>MGHHHHHHMKFGPETIIHGDCIEQMNALPEKSVDLIFADPPYNLQLGGDLLRPDNSKVDAVDDHWDQFESFAAYDKFTREWLKAARRVLKDDGAIWVIGSYHNIFRVGVAVQDLGFWILNDIVWRKSNPMPNFKGTRFANAHETLIWASKSQNAKRYTFNYDALKMANDEVQMRSDWTIPLCTGEERIKGADGQKAHPTQKPEALLYRVILSTTKPGDVILDPFFGVGTTGAAAKRLGRKFIGIEREAEYLEHAKARIAKVVPIAPEDLDVMGSK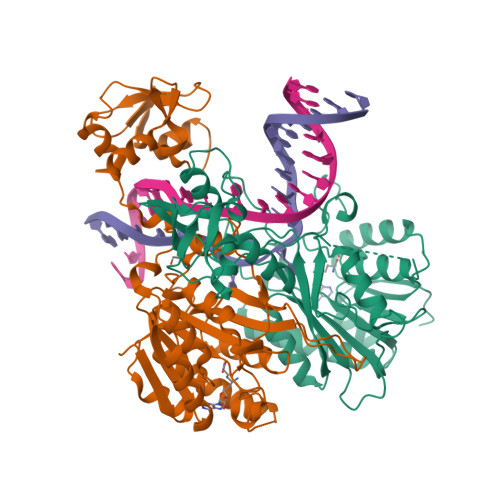RAEPRVPFGTIVEAGLLSPGDTLYCSKGTHVAKVRPDGSITVGDLSGSIHKIGALVQSAPACNGWTYWHFKTDAGLAPIDVLRAQVRAGMN[2x]> MARAYSLLSSRNRLIPRVEVQCRKREWVKTD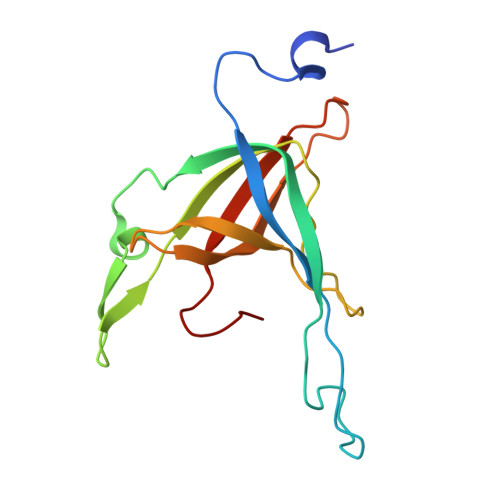PDSPFLNGGREVLYTPFTAVECTVQPMRGKAIRDQNNQLMIGGEEDYDSYTVYSETLLFRAREGTEHLSDQMLLPDSGGGQTWFTVMKADMYPSSGVPRYRYYLIAVPVGTEGGL>[2x]SHNDKDLSTWQTFRRLWPTIAPFK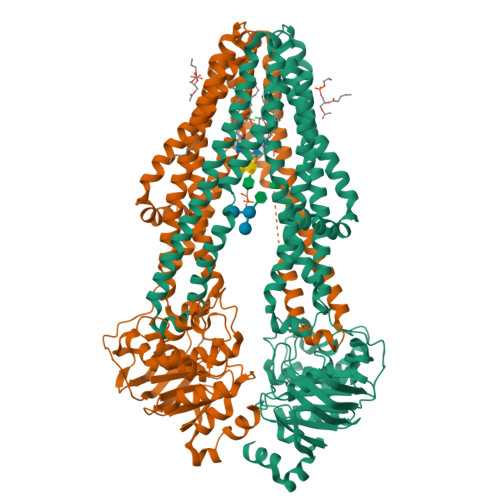AGLIVAGVALILNAASDTFMLSLLKPLLDDGFGKTDRSVLVWMPLVVIGLMILRGITSYVSSYCISWVSGKVVMTMRRRLFGHMMGMPVSFFDKQSTGTLLSRITYDSEQVASSSSGALITVVREGASIIGLFIMMFYYSWQLSIILIVLAPIVSIAIRVVSKRFRNISKNMQNTMGQVTTSAEQMLKGHKEVLIFGGQEVETKRFDKVSNRMRLQGMKMVSASSISDPIIQLIASLALAFVLYAASFPSVMDSLTAGTITVVFSSMIALMRPLKSLTNVNAQFQRGMAACQTLFTILDSEQEKDEGKRVIERATGDVEFRNVTFTYPGRDVPALRNINLKIPAGKTVALVGRSGSGKSTIASLITRFYDIDEGEILMDGHDLREYTLASLRNQVALVSQNVHLFNDTVANNIAYARTEQYSREQIEEAARMAYAMDFINKMDNGLDTVIGENGVLLSGGQRQRIAIARALLRDSPILILDEATSALDTESERAIQAALDELQKNRTSLVIAHRLSTIEKADEIVVVEDGVIVERGTHNDLLEHRGVYAQLHKMQFGQ> GSNRRLQQTQAQVDEVVDIMRVNVDKVLERDQKLSELDDR;> MALSEIETRHSEIIKLENSIRELHDMFMDMAMLVESQGEMIDRIEYNVEHAVDYVERAVSDTKKAVK;> MRNELEEMQRRADQLADESLESTRRMLQLVEESKDAGIRTLVMLDEQGEQLDRVEEGMNHINQDMKEAEKNLKDLGK;> MARENEMD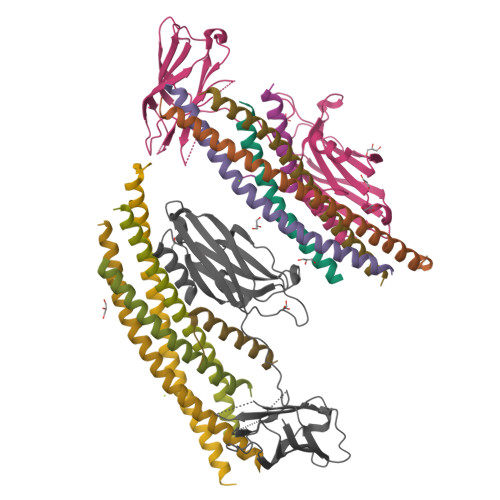ENLEQVSGIIGNLRHMALDMGNEIDTQNRQIDRIMEKADSNKTRIDEANQRATKMLG;> MEFVMKQALGGATKDMGKMLGGDEEKDPDAAKKEEERQEALRQAEEERKAKYAKMEAEREVMRQGIRDKYGIKKKEEREAEAQ;> EKLGKLQYSLDYDFQNNQLLVGIIQAAELPALDMGGTSDPYVKVFLLPDKKKKFETKVHRKTLNPVFNEQFTFKVPYSELGGKTLVMAVYDFDRFSKHDIIGEFKVPMNTVDFGHVTEEWRDLQSAEKEEQEKLGDICFSLRYVPTAGKLTVVILEAKNLKKMDVGGLSDPYVKIHLMQNGKRLKKKKTTIKKNTLNPYYNESFSFEVPFEQIQKVQVVVTVLDYDKIGKNDAIGKVFVGYNSTGAELRHWSDMLANPRRPIAQWHTLQVEEEVDAMLAVKK Profilin is an ubiquitous cytoskeletal protein that interacts with several molecules, such as actin, proline-rich ligands, and phosphoinositides to perform several cellular functions. Profilin is also an important allergen present in pollen grains, food plants, and rubber tree, and it is considered a pan-allergen, because it is present in all eukaryotic cells and is therefore involved in allergic cross-reactions. In this work, we focus on the study of two plant pan-allergens, profilins from the rubber tree (rHev b 8) and maize (rZea m 12), in their monomeric and dimeric forms. Here we isolated the monomeric and dimeric species of the recombinant profilin allergens rHev b 8 and rZea m 12 and obtained their crystallographic 3D structures.

The rHev b 8 and rZea m 12 crystals (5 mg/mL) were obtained using the conditions described in the materials and methods section. These crystals diffracted to resolutions of 1.9 and 2.2 Å, respectively, and belonged to the P43212 space group. A backbone alignment of the two 3D-structures reveals that they adopt the same conformation, with a root-mean-square-deviation (rmsd) of 0.27 Å. The sequence alignment shows that the principal differences are between residues 37ANFPQFKSEEITGIMSDFH55for rHev b 8 and 37ENFPELKPEEVAGMIKDFD55 for rZea m 12. These residues are structurally located in a region exposed to the solvent, mainly in the loop that connects β-strand 2 and α-helix 2, but some also belong to α-helix 2. The electrostatic potential surfaces of both structures display the most significant differences that lead to a more electronegative surface on rZea m 12. In general, the most important structural differences between rHev b 8 and rZea m 12 are the contributions of some side-chains that alter the surface charge, essentially at the loop that has been considered important for antibody recognition 262728 and it is exposed on the surface of the dimer structure. The assays showed that mAb 2F5 specifically recognizes monomeric rHev b 8, even at a low concentration (2 μg/mL); conversely, mAb 2F5 showed no reactivity towards monomeric rZea m 12, suggesting that this IgE recognizes a conformational epitope on the surface of rHev b 8 that is not shared with rZea m 12. From the immunological standpoint, it is relevant to note that mAb 2F5 only recognized rHev b 8, but not rZea m 12, even though the sequence identity is 79.4% and the folding is very similar (rmsd of 0.27 Å for Cα).

> GMSWQAYVDDHLLCDIEGQHLSAAAIVGHDGSVWAQSENFPELKPEEVAGMIKDFDEPGTLAPTGLFVGGTKYMVIQGEPGVVIRGKKGTGGITIKKTGMSLIIGIYDEPMTPGQCNMVVERLGDYLIEQGF>MSCPVPACCALLLVLGLCRARPRNALLLLADDGGFESGAYNNSAIATPHLDALARRSLLFRNAFTSVSSSSPSRASLLTGLPQHQNGMYGLHQDVHHFNSFDKVRSLPLLLSQAGVRTGIIGKKHVGPETVYPFDFAYTEENGSVLQVGRNITRIKLLVRKFLQTQDDRPFFLYVAFHDPHRCGHSQPQYGTFCEKFGNGESGMGRIPDWTPQAYDPLDVLVPYFVPNTPAARADLAAQYTTVGRMDQGVGLVLQELRDAGVLNDTLVIFTSDNGIPFPSGRTNLYWPGTAEPLLVSSPEHPKRWGQVSEAYVSLLDLTPTILDWFSIPYPSYAIFGSKTIHLTGRSLLPALEAEPLWATVFGSQSHHEVTMSYPMRSVQHRHFRLVHNLNFKMPFPIDQDFYVSPTFQDLLNRTTAGQPTGWYKDLRHYYYRARWELYDRSRDPHETQNLATDPRFAQLLEMLRDQLAKWQWETHDPWVCAPDGVLEEKLSPQCQPLHNELRSHHHHHH[8x]

Mucopolysaccharidosis type IIIA (MPS IIIA) is caused by the functional defect of N-sulfoglucosamine sulfohydrolase (SGSH; also known as sulfamidase, sulfamate sulfohydrolase and heparan N-sulfatase; EC 3.10.1.1) and represents one of the most frequent lysosomal storage diseases worldwide. SGSH belongs to the sulfatase family and catalyses the cleavage of N-linked sulfate groups from the GAGs heparan sulfate and heparin. The leading cysteine is post-translationally converted to a formylglycine (FGly) residue, which is crucial for the catalytic process. Despite the low sequence identity between this unique N-sulfatase and the group of O-sulfatases, they share a similar overall fold and active-site architecture, including a catalytic formylglycine, a divalent metal-binding site and a sulfate-binding site.

Two crystal forms of glycosylated SGSH were grown at different pH values. The form grown at pH 5.1 is designated crystal form L (large unit cell). Its structure was refined to 2.40 Å resolution. There are two molecules in the asymmetric unit of crystal form S and eight molecules in that of form L. The enzyme appears to exist as a homodimer in both crystal forms. Since the SGSH structure was determined in two crystal forms, S and L, we could use the ten crystallographically independent monomers of SGSH to assess the structural flexibility of the enzyme under two different crystallization conditions. The enzyme subunits display a low rigid-body structural flexibility in the S form (Cα r.m.s.d. of 0.20 Å between the two chains, with NCS restraints) as well as the L form (r.m.s.d. ranging from 0.10 to 0.17 Å, with NCS restraints). To investigate the mobility at the dimer interface, all five homodimers were superimposed based on one of the subunits in each dimer. The relative orientation of the dimer subunits in the L form differs from that in the S form by 2.6–3.0°, indicating that the dimer interface is slightly flexible, possibly owing to crystal packing. Ten chains of SGSH monomers found in the two crystal forms in the current study associate to form five homodimers. However, the dimer interface is slightly flexible, displaying a rotation of up to 3.0° in the two crystal forms.>MDSLAESRWPPGLAVMKTIDDLLRCGICFEYFNIAMIIPQCSHNYCSLCIRKFLSYKTQCPTCCVTVTEPDL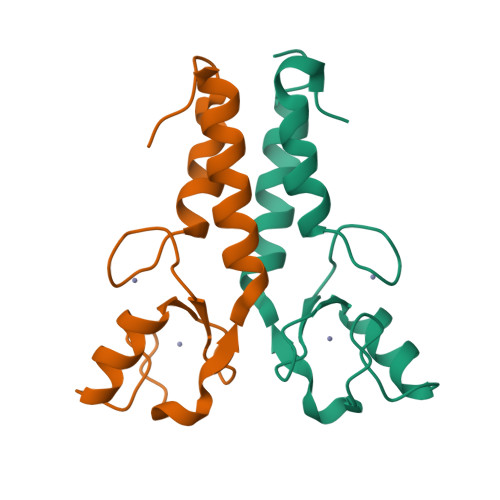KNNRILDELVKSLNFARNHLLQFALES[2x]> MDRALFLAMSGAKQNMQALQLRANNLANVSTTGFRADLAQARSMQAYGEGHPSRVFSMTERPGHNFAQGSVITTGRDLDVTIEGSGWISVLDHTGKEGLTRNGNLKVDQNGMLTNASGHLVLGENDAPITLPIPLSKIEIGRDGTISVLPQGAPAEEFQAVDRIKLVKPNDQSLFKDTNGLFRHKTPNQPYEADATVSLQTGAIEGSNVNAVGEMTALIDLQ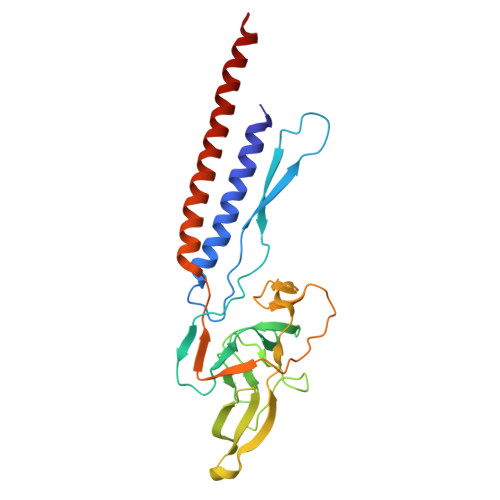RQFEMQVKMMSTAEEMDKSSDSLLRMS>[2x]MI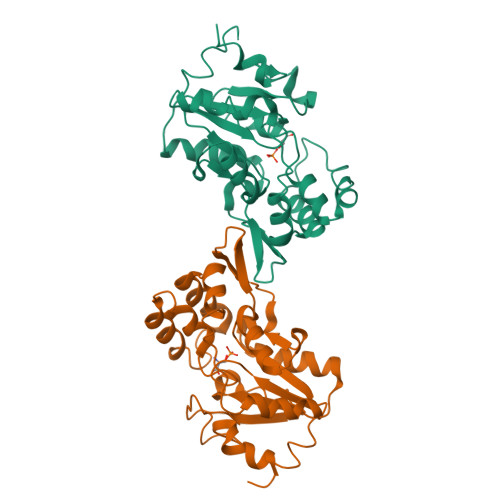SHSELRKLFYSADAVCFDVDSTVIREEGIDELAKICGVEDAVSEMTRRAMGGAVPFKAALTERLALIQPSREQVQRLIAEQPPHLTPGIRELVSRLQERNVQVFLISGGFRSIVEHVASKLNIPATNVFANRLKFYFNGEYAGFDETQPTAESGGKGKVIKFLKEKFHFKKIIMIGDGATDMEACPPADAFIGFGGNVIRQQVKDNAKWYITDFVELLGELEE>[4x]MASWSHPQEKGALEVLFQGPMKFSNITIKNFRNFEKVNINLDNKNVIFGMNDIGKTNFLYALRFLLDKEIRKFGFNKSDYHKHDTSKKIEIILTLDLSNYEKDEDTKKLISVVKGARTSANADVFYIALESKYDDKELYGNIILKWGSELDNLIDIPGRGNINALDNVFKVIYINPLVDLDKLFAQNKKYIFEESQGNESDEGILNNIKSLTDQVNQQIGEMTIIKGFQQEITSEYRSLKKEEVSIELKSEMAIKGFFSDIIPYIKKDGDSNYYPTSGDGRRKMLSYSIYNYLAKKKYEDKIVIYLIEEPEISLHRSMQIALSKQLFEQSTYKYFFLSTHSPELLYEMDNTRLIRVHSTEKVVCSSHMYNVEEAYGSVKKKLNKALSSALFAERVLLIEGPSEKILFEKVLDEVEPEYELNGGFLLEVGGTYFNHYVCTLNDLGITHIIKTDNDLKSKKGKKGVYELLGLNRCLNLLGRENLDEITIDIPEDIKGKKKKERLNERKKEIFKQYKNEVGEFLGERIYLSEIDLENDLYSAIGESMKRIFENEDPVHYLQKSKLFNMVELVNNLSTKDCFDVFEHEKFACLKELVGSDRG;>MSREQIIKDGGNILVTAGAGSGKTTILVSKIEADLKENKTHYSIAAVTFTNKAAKEIEGRLGYSSRGNFIGTNDGFVESEIIRPFIKDAFGNDYPDNFTAEYFDNQFASYDKGLQVLKYQNILGTYSNPKKNFKFQLALDILKKSLVARQYIFSKYFKIFIDEYQDSDKDMHNLFMYLKDQLKIKLFIVGDPKQSIYIWRGAEPENFNGLIENSTDFNKYHLTSNFRCCQDIQNYSNLFNEETRSLIKEKNEVQNVISIADDMPISDILLKLTEEKQVLNIEAELVILVRRRNQAIEIMKELNEEGFNFIFIPQTPLDRATPNATLLKEVIKYVKNDRYSIYDLAAEIVGNLSSREIKEIQKIINELLVPNINQVLINQVLINLFAKLEITLDTREITAFTEVMMTNEFDIAFDTNEYLHKIFTVHSAKGLEFNQVIITASDYNVHYNRDTNEHYVATTRAKDKLIVIMDNKKYSDYIETLMKELKIKNIIKSI[4x]

The Gabija system is a newly discovered bacterial immune system that consists of GajA and GajB. GajA is an OLD nucleases family protein, while GajB belongs to the SF1 helicases. The Gabija complex has sequence-specific DNA nuclease activity and prefers circular rather than linear DNA as substrate, its activity is more sensitive to concentrations change of nucleotides compared to GajA alone. Our data suggest a mechanism of Gabija immunity: the nuclease activity of Gabija complex is inhibited under physiological conditions, while it is activated by depletion of NTP and dNTP upon the replication and transcription of invading phages and cleave the circular DNA to prevent phage DNA replication.

Here we report the cryo-EM structure of the Gabija complex from Bacillus cereus VD045 at 3.6 Å, which provides the direct evidence of interactions between GajA and GajB. The resolved structure shows that the Gabija complex adopts an octameric ring structure with four GajA and four GajB. The whole Gabija complex resembles an octameric ring with three 2-fold symmetry axes. The three dimensions of the octameric ring are 171 Å × 143 Å × 91 Å; The inner diameter of the ring is 35 Å at the narrowest region. SEC-MALS results show that individual GajA and GajB exist in the form of tetramer and monomer respectively, supporting the hypothesis that the octameric ring of Gabija complex is formed though two steps: the tetramer formation of GajA and subsequent octamer formation of Gabija complex. The interactions within GajA1-GajB1 are mediated by the ATPase domain of GajA and the 1A, 1B domains of GajB. Despite being present in the cryo-EM protein sample, domain 2A and 2B could not be traced in the electron density map, demonstrating that this region is quite flexible in the Gabija complex. Size exclusion chromatography demonstrates that the NTR region of GajB indeed binds to GajA, while the CTR region of GajB doesn’t bind to GajA. There is a highly conserved region (E379, E383, D432, D434, D511, D513, K541) in the Toprim domain. Non-specific DNA cleavage activity is only detected in the GajAmut1. These data suggest that the lysine-rich basic patch 1 of loop (residue 436-442) is responsible for the selection of sequence specific DNA digestion of GajA.>[8x]CNMKQEQMRLANQLCFSAYNVSRLFAQFYEKKLKQFGITYSQYLVLLTLWEENPQTLNSIGRHLDLSSNTLTPMLKRLEQSGWVKRERQQSDKRQLIITLTDNGQQQQEAVFEAISS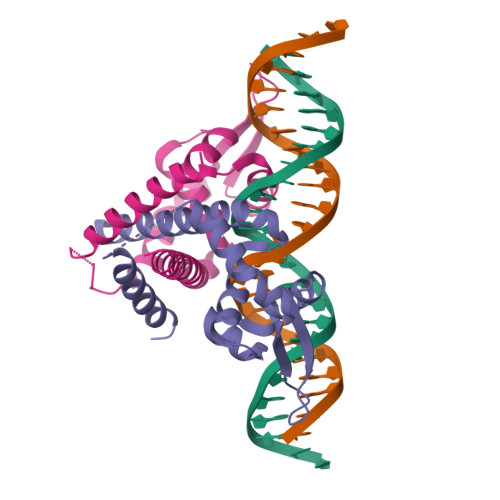CLPQEFDTTEYDETKYVFEELEQTLKHLIEK>SNAMDILRKGNKDLIKDINRYTVLNLIREKGEITRTEIAKKCDFGMSTLTYILDDLQQEGIILEGAETSSTGGRRAKLVRFNKDYGFVVSVKVEEEQLLFALTDLNAEIIENTSIPFSSEKKPEEAIELIAKNVKKMCGNRDMNHLLGVGIAISGLVNRKKGTVIRSTMLGWENVALEAMLHAHFPDIPVYVDKNINCYTLAELWLGEGKQSNNFATVSVGAGLGLSVVINRQIYYGAQGGAGEFGHTTIQPGGYKCHCGQKGCLEMYASEFYFRNRGEELKEAYPTSELNDFHFDKVAKSA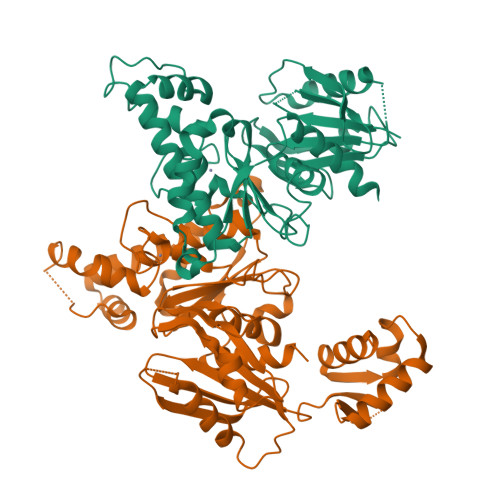RAGDEMATELMGKMGEYLGYGIRNIINTFNPEKVIIVGEGLHHRDLFLTKIDEIASQNFFSGAGFETEITTTSLEDPAWLQGAALLVIHQLFQVPIYEEEQTLLR[2x]(2R,4S,5R,6R)-4-amino-5-hydroxy-6-methyltetrahydro-2H-pyran-2-yl [(2R,3S,5R)-3-hydroxy-5-(5-methyl-2,4-dioxo-3,4-dihydropyrimidin-1(2H)-yl)tetrahydrofuran-2-yl]methyl dihydrogen 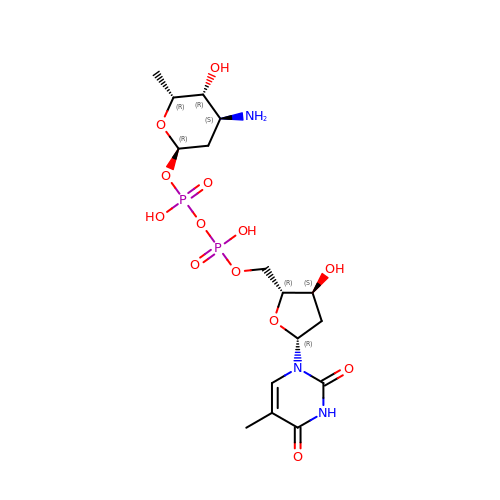diphosphate | C16 H27 N3 O13 P2 | CEQVCLWWGAYCPR-RIBQXPMZSA-N>MAKFFIDRPIFAWVISIFIIAAGIFGIKSLPVSQYPSVAAPTITLHAIYPGASAQVMEGSVLSVIERNMNGVEGLDYMSTSADSSGSGSVSLTFTPDTDENLAQVEVQNKLSEVLSTLPATVQQYGVTVSKARSNFLMIVMLSSDVQSTEEMNDYAQRNVVPELQRIEGVGQVRLFGAQRAMRIWVDPKKLQNYNLSFADVGSALSAQNIQISAGSIGSLPAVRGQTVTATVTAQGQLGTAEEFGNVILRANTDGSNIYLKDVAKVGLGMEDYSSSTRLNGVNTTGMAVMLSNSGNAMATAKAVKERLAVLEKYFPQGMSWKTPYDTSKFVEISIEKVIHTLIEAMVL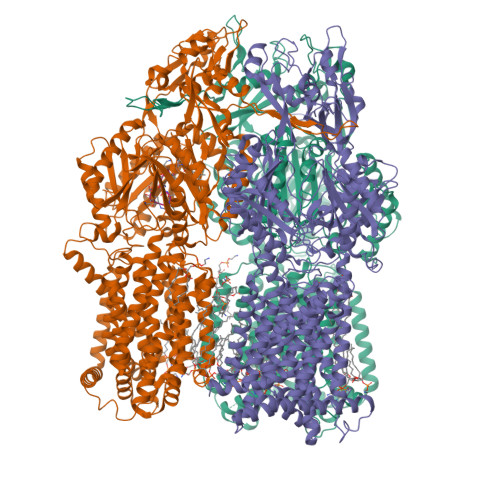VFVVMYLFLQNIRYTLIPTIVVPISLLGGFAFISYMGMSINVLTMFAMILVIGIVVDDAIVVVENVERIMAGEGLPPKEATKKAMGQISGAVIGITAVLISVFVPLAMFSGAAGNIYKQFALTMASSIAFSAFLALTLTPALCATMLKTIPKGHHEEKKGFFGWFNKKFDSWTHGYEGRVAKVLRKTFRMMVVYIGLAVVGVFLFMRLPTSFLPTEDQGFVMVSVQLPAGATKERTDATLAQVTQLAKSIPEIENIITVSGFSFSGSGQNMAMGFAILKDWNERTASGSDAVAVAGKLTGMMMGTLKDGFGIAVVPPPILELGNGSGLSINLQDRNNTGHTALLAKRNELIQKMRASGLFDPSTVRAGGLEDSPQLKIDINRAAAAAQGVSFADIRTALASALSSSYVSDFPNQGRLQRVMVQADGDARMQPADILNLTVPNSSGIAVPLSSIATVSWQMGTEQSVRFNGYPAMELSGSPATGVSTGQAMEAVQKMVDELGSGYSLEWGGQSREEAKGGSQTIALYALAAVAVFLVLAALYESWSIPLAVLLVMPLGLAGAAAGVTGRNLFEGLLGSVPSFANDIYFQVGFVTVMGLSAKNAILIIEFAKDLQAQGKSAVEAALEAARLRFRPIIMTSFAFILGVVPLYIAGGASSASQRAIGTTVFWGMLIGTLLSVFLVPLFYVVVRKFFKETAHE[3x];> XATAAALLAAT> TGTAGDLASLLAGDGLGRKSKAWRVLRAQQQACGEGSGEEGEITEIEGLGLGEGMEGFERELDNIPDTLPDDERLALWKGKLKHYLILSSAGKPIWSRHGDLSLVNSTMGVVQTIISFYEGARNPLLGFTAGKVRFVILIKGPLYFVAISRLRESDAQLRAQLEALYMQILSTLTLPILTNIFAHRPSTDLRGPLQGTESLLASLADSFTKGSPSTLLSALECLRLRKSQRQAITNIFLKSRCEELLYGLLVAGGKLVSVIRPRKHSLHPSDLQLIFNMLFESGGIKGNGGENWIPLCLPAFNNTGYLYMYVSFLDDKAPDDQNQPPESSNLDASNKNSSNTPDDDLTALILISPSREAFYALQSMRTRLVSQLLSTGYLSLIRSTALSGRPSITSILPKTPLLHFLYKSRPNVQWCMSSLSSLTPPGATATETLLARRKLMSVYEELHAALHARHAHLRVVYSTADEKEGEGLACLGWSTPAFEVYCVAPGCVGRAGMAREVNRVVQWARREEERLFILGGGVF;> MTTPVSPSPSGIIPAQLGFLAIYNPALGTTDETLEDQIVYYATASTLSQARRRHRRPRRRDRQRAQSVVKDSRPNAAGATGDSEAVAEDKDPVSKEERHERLRQIGLAQGMVEFAKSFSDGEPVDTIDTEKARVILVEVEEGWWILASIDLTRLPLPQIKTPTSSSAPPPAPNLNPLPPEPAYEYSSREVKPPSLLRADLLRAYDLFLLHHGSSLSSLLASQGRAQLVASLTRFWDHFLATWNVLLHGNPACDVFGGIKLAASGELGIGVGEEERGSGEREVLEGLVERVEGLVDVVVGRYGGPPSEKGPEEEQWLGLGGEVGEEDGAVFLGVGALDRKSLRGVVQWMEEVYVWGENAFGKPRRDLSTGHFLLGL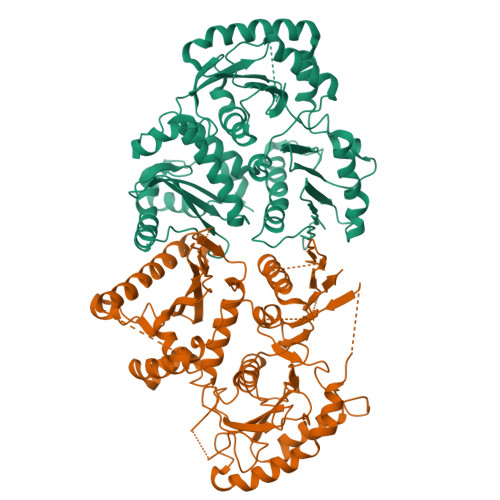SECSEEELTSSQANPKAIFVELKPSYQHPSRKIPPEDPQPLGKVGPELPRDHTARLRPVIYVSQPFIYILLFSEITPSPSTWPTLAESLHAQLSPLQKPLLHSTSYRPERPVVETTSSSGTTTQHQIFDLVYDTETLTLQSTIPNIPDPFPYSATTPTGHSTGQQHHQQSIWTRVEALQTHAQILAILSSGRAIPTDPSSFTHLPWEEGERTCKTARGWWIVWTRVVEHSPPDAVSLHHARDDDDNDDDASCSVLGHLRSVSSSHAAGSTSSSSGSGFGLGAIPGLGGLGGWAADGATRLAQGIGIDTRRYVEGLLTSLGR>[2x]MNNDVFPNKFKAALAAKQVQIGCWSALSNPISTEVLGLAGFDWLVLDGEHAPNDISTFIPQLMALKGSASAPVVRVPTNEPVIIKRLLDIGFYN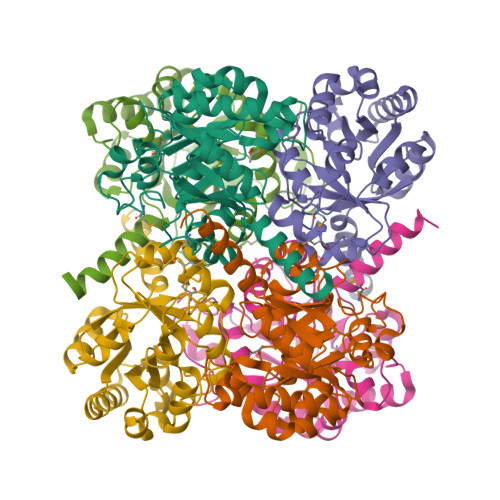FLIPFVETKEEAELAVASTRYPPEGIRGVSVSHRANMFGTVADYFAQSNKNITILVQIESQQGVDNVDAIAATEGVDGIFVGPSDLAAALGHLGNASHPDVQKAIQHIFNRASAHGKPSGILAPVEADARRYLEWGATFVAVGSDLGVFRSATQKLADTFKK6-methylpyridine-3-carboxamide 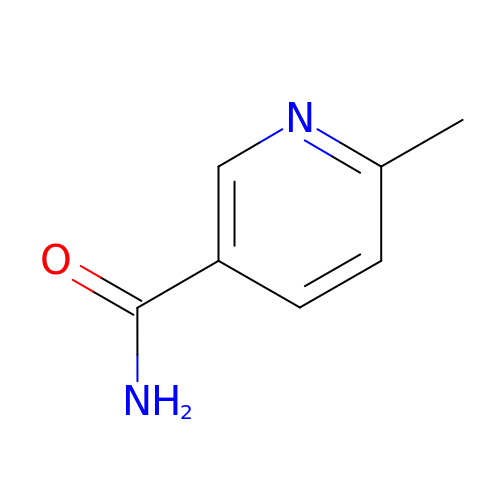| C7 H8 N2 O | IJXDURUAYOKSIS-UHFFFAOYSA-N>AUGUGGCAU[28x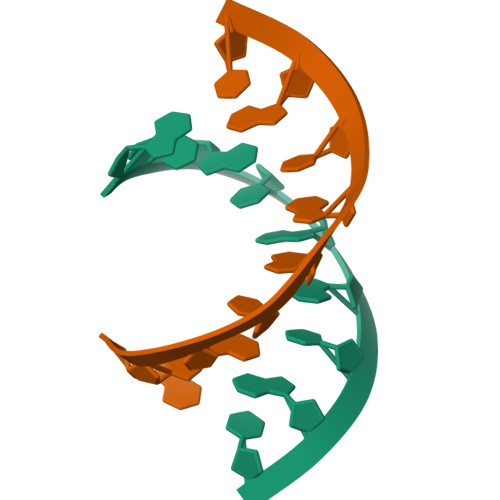]>[2x]MNKFKGNKVVLIGNGAVGSSYAFSLVNQSIVDELVIIDLDTEKVRGDVMDLKHATP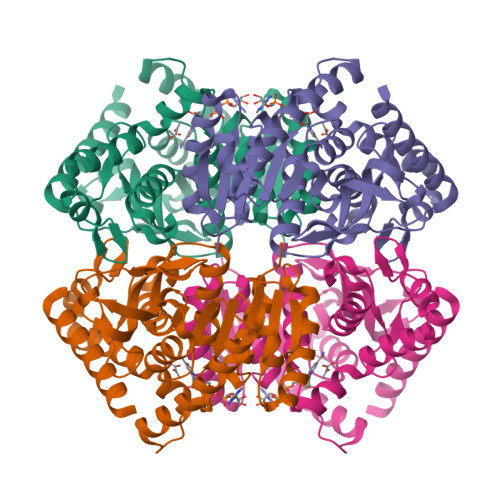YSPTTVRVKAGEYSDCHDADLVVICAGAAQKPGETRLDLVSKNLKIFKSIVGEVMASKFDGIFLVATNPVDILAYATWKFSGLPKERVIGSGTILDSARFRLLLSEAFDVAPRSVDAQIIGEHGDTELPVWSHANIAGQPLKTLLEQRPEGKAQIEQIFVQTRDAAYDIIQAKGATYYGVAMGLARITEAIFRNEDAVLTVSALLEGEYEEEDVYIGVPAVINRNGIRNVVEIPLNDEEQSKFAHSAKTLKDIMAEAEELK> MGSSHHHHHHSQDPNSLEVLFQGPMAGGRDRGDLAARQLVFLLPEHLKDASKKKKKSSLLFVKLANPHSGEGATYLIDMCLQQLFEIKVFKEKHHSWFINQSVQSGGLLHFATPMDPLFLLLHYL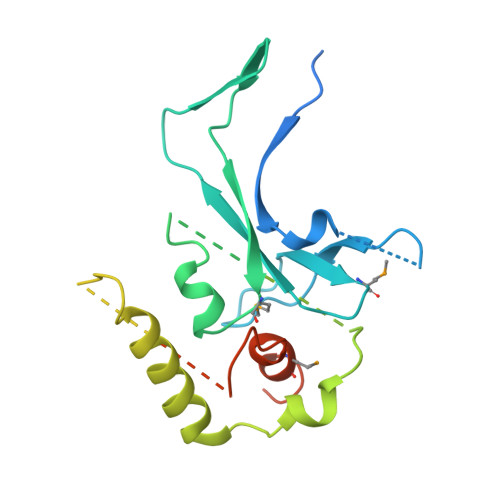LKAGKEGKYQPLDQVVVDDTFPDCTLLLRFPELEKSLRHVTEEKEVNSKKYYKYSSEKTLKWLEKKVNQTVVALKANNVNVGARVQSSAYFSGGQVSRDKEEDYVRYAHGLISDYIPKELSDDLSKFLKLPEPPASLPNPPSKKLKLSDEPVEAKEDYTKFNTKDLKTGKKNSKMTAAQKALAKVDKSGMKSIDAFFGAKNKKTGKI>[2x]MAHHHHHHMKSFKVALAQFSPHIGNIDSNTQKMIEQANQAKKQDADLIIFPELSVIGYPAEDLLLRPNLNKRMQKAFAQLSEVKDIVMVFGFVNQTEDGQRYNSAAVMKDGQVLGVFNKHNLPNYGVFDEKRYFQKGHQHLVFEYLGHKFGVLICEDIWSINTVKQLSQLNVDTVLVLNSSPYEVGKPQHRKQTLSELAKQLHLNIVYVNQVGGQDDLIFDGTSFVSNQNGEIALQAPSFKEDLYIAEFDRDTKLYKVVESAPALETFAEIYQGLVMATRDYVERSGFPGVILGLSGGIDSALTLAIAVDAIGAERVQAVMMPYTYTSQISVEDAAEQARRMGVTFGIAEIHSIVNSFMQTLYPFFGNSPADATEENLQARARGTLLMGLSNKFGNLVLSTGNKSELSVGYCTLYGDMVGGFAVLKDVYKTIVFELAKYRNSLSETPVIPERVITRPPSAELRPDQKDQDSLPAYDVL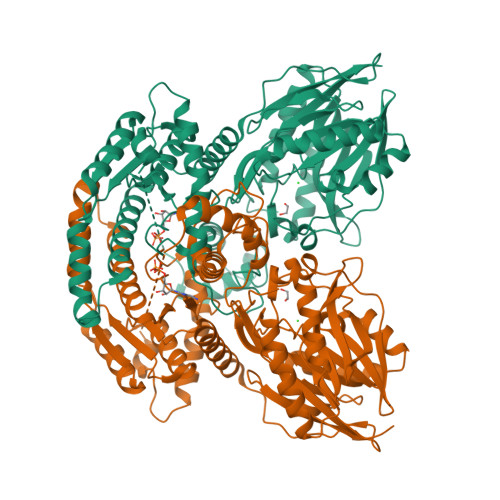DAILYAYIEEDLGQADIIAKGFDKEVVEKVIRLVDRNEYKRRQGAIGPRITSRAFSRERRYPIVNGWTAND Vertebrates possess a second DCTD-like protein, CDADC1 (NYD-SP15). Unlike DCTD, CDADC1 contains two CMP/dCMP-like deaminase domains (IPR002125), connected by a long (>100 residues) linker within a single polypeptide chain, resulting in CDADC1 being approximately triple the length of DCTD (e.g. 514 residues in human CDADC1 versus 178 in human DCTD). The C-terminal deaminase domain (CTD) of CDADC1 contains a potentially active HAE motif, but its N-terminal domain (NTD) appears to be naturally inactivated due to the mutation of the proton shuttle glutamate (the HAG motif instead of HAE), suggesting noncatalytic function. In this work, we provide biochemical and structural evidence that human CDADC1 deaminates dCTP and CTP.

CDADC1 hexamers are formed by symmetric stacking of two trimers, i.e. trimers face each other with the same sides. CDADC1 apo hexamers are less tight than trimers, with a contact area per protomer of ~270 Å2. Each protomer from one trimer interacts with two protomers from the other trimer. With one of them, it is arranged in an antiparallel symmetric manner. However, no direct contacts can be seen between the two protomers in the apo model. One potential contact point between the pair is the “blob” in the map where two trimers are the furthest from each other (~7 Å), between two C197. The blob is likely derived from the partially structured 1–28 region. The interaction with the second protomer is more direct. It is achieved by symmetric hydrogen bonds between guanidino groups of R185 and carbonyl oxygens of A186, located between Nα4 and Nβ5 of the NTD. Therefore, we conclude that this interaction is likely the dominant force for hexamer formation in the absence of substrate, which highlights the important role played by Nα4 in both trimer and hexamer formation.

>[6x]MGSSHHHHHHSSGLVPRGSHMKEAGQMQNLESARAGRSVSTQTGSMTGQIPRLSKVNLFTLLSLWMELFPAEAQRQKSQKNEEGKHGPLGDNEERTRVSTDKRQVKRTGLVVVKNMKIVGLHCSSEDLHAGQIALIKHGSRLKNCDLYFSRKPCSACLKMIVNAGVNRISYWPADPEISLLTEASSSEDAKLDAKAVERLKSNSRAHVCVLLQPLVCYMVQFVEETSYKCDFIQKITKTLPDANTDFYYECKQERIKEYEMLFLVSNEEMHKQILMTIGLENLCENPYFSNLRQNMKDLILLLATVASSVPNFKHFGFYRSNPEQINEIHNQSLPQEIARHCMVQARLLAYRTEDHKTGVGAVIWAEGKSRSCDGTGAMYFVGCGYNAFPVGSEYADFPHMDDKQKDREIRKFRYIIHAAQNALTFRCQEIKPEERSMIFVTKCPCDECVPLIKGAGIKQIYAGDVDVGKKKADISYMRFGELEGVSKFTWQLNPSGAYGLEQNEPERRENGVLRPVPQKEEQHQDKKLRLGIH> GSHMH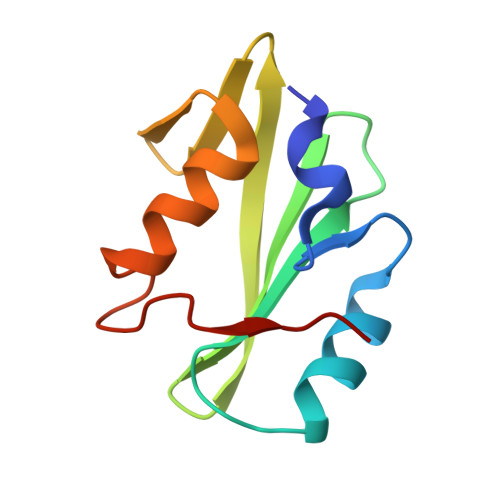ESKEWYHASLTRAQAEHMLMRVPRDGAFLVRKRNEPNSYAISFRAEGKIKHCRVQQEGQTVMLGNSEFDSLVDLISYYEKHPLYRKMKLRYPINEE> MASDYKDDDDKRRRGMEGAKLSAVRIAVREAPYRQFLGRREPSVVQFPPWSDGKSLIVDQNEFHFDHAFPATISQDEMYQALILPLVDKLLEGFQCTALAYGQTGTGK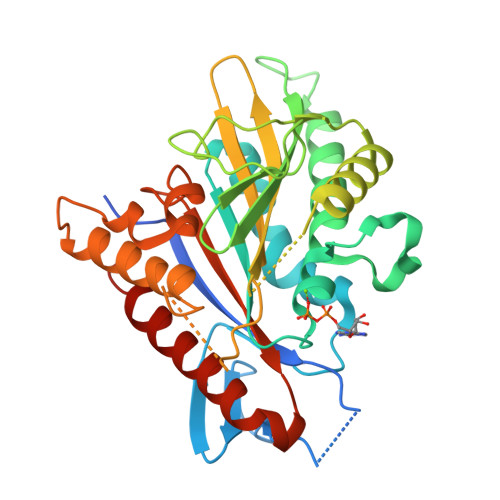SYSMGMTPPGEILPEHLGILPRALGDIFERVTARQENNKDAIQVYASFIEIYNEKPFDLLGSTPHMPMVAARCQRCTCLPLHSQADLHHILELGTRNRRVRPTNMNSNSSRSHAIVTIHVKSKTHHSRMNIVDLAGSEGVRRTGHEGVARQEGVNINLGLLSINKVVMSMAAGHTVIPYRDSVLTTVLQASLTAQSYLTFLACISPHQCDLSETLSTLRFGTSAKAAALEHHHHHH2-[4-({[4-(ethylsulfonyl)phenyl]acetyl}amino)phenyl]-2-methyl-N-phenylpropanamide 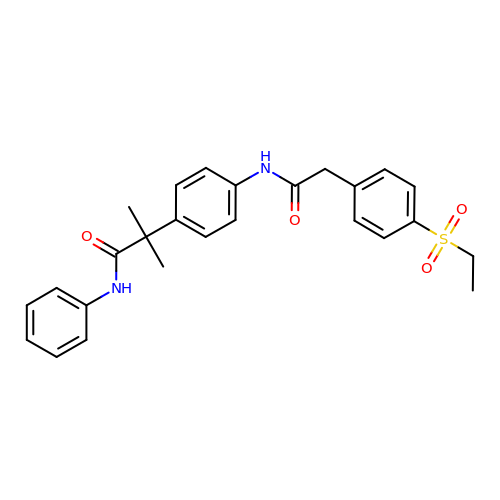| C26 H28 N2 O4 S | QECSHZAJHGHAOA-UHFFFAOYSA-N> MLRVFILYAENVHTPDTDISDAYCSAVFAGVKKRTKVIKNSVNPVWNEGFEWDLKGIPLDQGSELHVVVKDHETMGRNRFLGEAKVPLREVLATPSLSASFNAPLLDTKKQPTGASLVLQVSYTPLPGAVPLFPPPTPLEPSPTLPDLDVVADTGGEEDTEDQGLTGDEAEPFLDQSGGPGAPTTPRKLPSRPPPHYPGIKRKRSAPTSRKLLSDKPQDFQIRVQVIEGRQLPGVNIKPVVKVTAAGQTKRTRIHKGNSPLFNETLFFNLFDSPGELFDEPIFITVVDSRSLRTDALLGEFRMDVGTIYREPRHAYLRKWLLLSDPDDFSAGARGYLKTSLCVLGPGDEAPLERKDPSEDKEDIESNLLRPTGVALRGAHFCLKVFRAEDLPQMDDAVMDNVKQIFGFESNKKNLVDPFVEVSFAGKMLCSKILEKTANPQWNQNITLPAMFPSMCEKMRIRIIDWDRLTHNDIVATTYLSMSKISAPGGEIEEEPAGAVKPSKASDLDDYLGFLPTFGPCYINLYGSPREFTGFPDPYTELNTGKGEGVAYRGRLLLSLETKLVEHSEQKVEDLPADDILRVEKYLRRRKYSLFAAFYSATMLQDVDDAIQFEVSIGNYGNKFDMTCLPLASTTQYSRAVFDGCHYYYLPWGNVKPVVVLSSYWEDISHRIETQNQLLGIADRLEAGLEQVHLALKAQCSTEDVDSLVAQLTDELIAGCSQPLGDIHETPSATHLDQYLYQLRTHHLSQITEAALALKLGHSELPAALEQAEDWLLRLRALAEEPQNSLPDIVIWMLQGDKRVAYQRVPAHQVLFSRRGANYCGKNCGKLQTIFLKYPMEKVPGARMPVQIRVKLWFGLSVDEKEFNQFAEGKLSVFAETYENETKLALVGNWGTTGLTYPKFSDVTGKIKLPKDSFRPSAGWTWAGDWFVCPEKTLLHDMDAGHLSFVEEVFENQTRLPGGQWIYMSDNYTDVNGEKVLPKDDIECPLGWKWEDEEWSTDLNRAVDEQGWEYSITIPPERKPKHWVPAEKMYYTHRRRRWVRLRRRDLSQM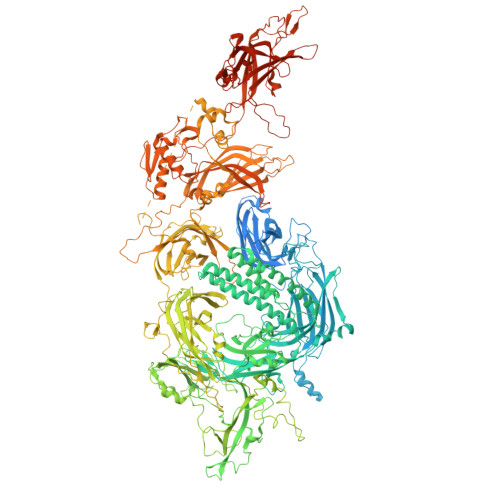EALKRHRQAEAEGEGWEYASLFGWKFHLEYRKTDAFRRRRWRRRMEPLEKTGPAAVFALEGALGGVMDDKSEDSMSVSTLSFGVNRPTISCIFDYGNRYHLRCYMYQARDLAAMDKDSFSDPYAIVSFLHQSQKTVVVKNTLNPTWDQTLIFYEIEIFGEPATVAEQPPSIVVELYDHDTYGADEFMGRCICQPSLERMPRLAWFPLTRGSQPSGELLASFELIQREKPAIHHIPGFEVQETSRILDESEDTDLPYPPPQREANIYMVPQNIKPALQRTAIEILAWGLRNMKSYQLANISSPSLVVECGGQTVQSCVIRNLRKNPNFDICTLFMEVMLPREELYCPPITVKVIDNRQFGRRPVVGQCTIRSLESFLCDPYSAESPSPQGGPDDVSLLSPGEDVLIDIDDKEPLIPIQEEEFIDWWSKFFASIGEREKCGSYLEKDFDTLKVYDTQLENVEAFEGLSDFCNTFKLYRGKTQEETEDPSVIGEFKGLFKIYPLPEDPAIPMPPRQFHQLAAQGPQECLVRIYIVRAFGLQPKDPNGKCDPYIKISIGKKSVSDQDNYIPCTLEPVFGKMFELTCTLPLEKDLKITLYDYDLLSKDEKIGETVVDLENRLLSKFGARCGLPQTYCVSGPNQWRDQLRPSQLLHLFCQQHRVKAPVYRTDRVMFQDKEYSIEEIEAGRIPNPHLGPVEERLALHVLQQQGLVPEHVESRPLYSPLQPDIEQGKLQMWVDLFPKALGRPGPPFNITPRRARRFFLRCIIWNTRDVILDDLSLTGEKMSDIYVKGWMIGFEEHKQKTDVHYRSLGGEGNFNWRFIFPFDYLPAEQVCTIAKKDAFWRLDKTESKIPARVVFQIWDNDKFSFDDFLGSLQLDLNRMPKPAKTAKKCSLDQLDDAFHPEWFVSLFEQKTVKGWWPCVAEEGEKKILAGKLEMTLEIVAESEHEERPAGQGRDEPNMNPKLEDPRRPDTSFLWFTSPYKTMKFILWRRFRWAIILFIILFILLLFLAIFIYAFPNYAAMKLVKPFS>[8x]MTHR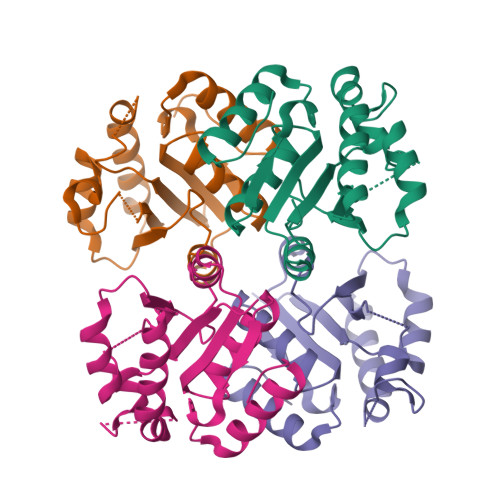ALLVVDYSYDFIADDGLLTCGKPGQNIEDFIVSRINDFNYYQDHIFFLMDLHYLHDIHHPESKLFPPHNIVDTSGRELYGKVGKLYETIKAQPNVHFIDKTRYDSFFGTPLDSLLRERSINQVEIVGVCTDICVLHTAISAYNLGYKISVPAEGVASFNQKGHEWALAHFKNSLGAEVEQHV>MTKPLDGINVLDFTHVQAGPACTQMMGFLGANVIKIERRGSGDMTRGWLQDKPNVDSLYFTMFNCNKRSIELDMKTPEGKELLEQMIKKADVMVENFGPGALDRMGFTWEYIQELNPRVILASVKGYAEGHANEHLKVYENVAQCSGGAAATTGFWDGPPTVSGAALGDSNSGMHLMIGILAALEIRHKTGRGQKVAVAMQDAVLNLVRIKLRDQQRLERTGILAEYPQAQPNFAFDRDGNPLSFDNITSVPRGGNAGGAGQPGWMLKCKGWETDADSYVYFTIAANMWPQICDMIDKPEWKDDPAYNTFEGRVDKLMDIFSFIETKFADKDKF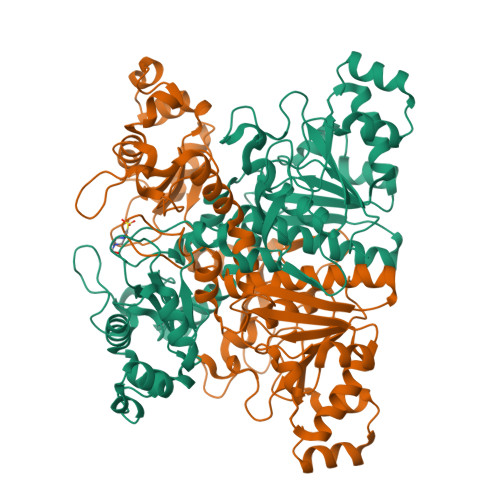EVTEWAAQYGIPCGPVMSMKELAHDPSLQKVGTVVEVVDEIRGNHLTVGAPFKFSGFQPEITRAPLLGEHTDEVLKELGLDDAKIKELHAKQVV[2x]>[2x]MDGSGEQPRGGGPTSSEQIMKTGALLLQGFIQDRAGRMGGEAPELALDPVPQDASTKKLSECLKRIRDELDSNMELQRMIAAVDTDS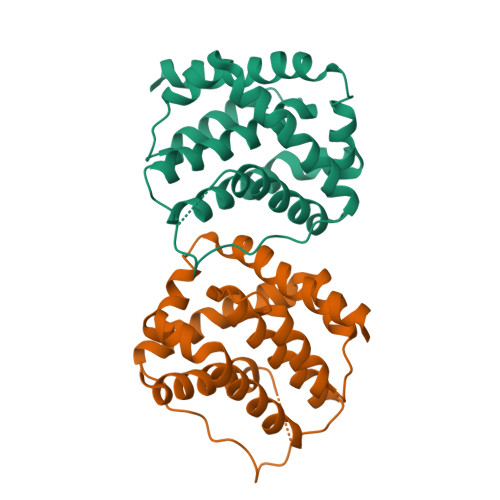PREVFFRVAADMFSDGNFNWGRVVALFYFASKLVLKALCTKVPELIRTIMGWTLDFLRERLLGWIQDQGGWDGLLSYFGTPTWQTVTIFVAGVLTASLTIWKKMG> XGPPGPPGDKGD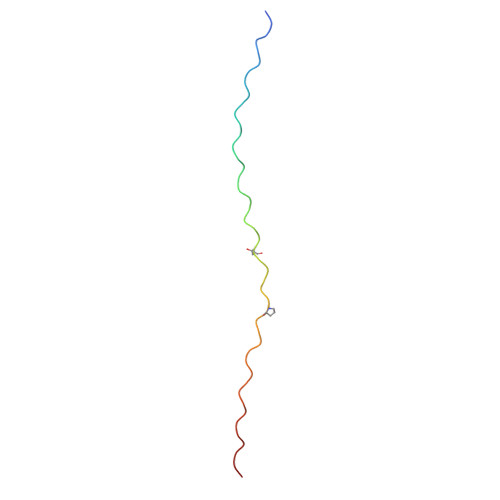KGPPGPPGARGEPGNIGFPGPPGPPGDKGDKGPPG(3R)-3-(4-methoxyphenyl)piperidine-2,6-dione 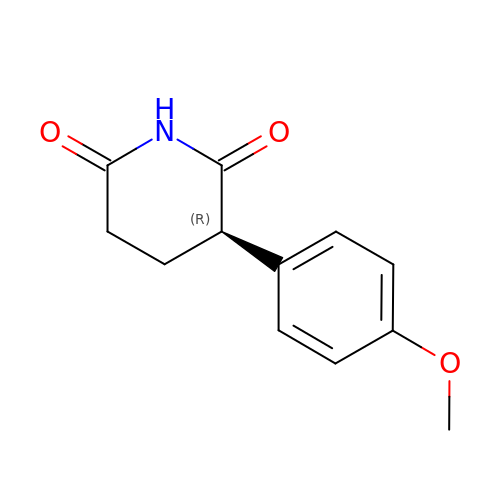| C12 H13 N O3 | UTEUBBDWRDGRCU-SNVBAGLBSA-N TDP-43 (TAR DNA-binding protein) is a DNA- and RNA-binding protein highly conserved in eukaryotes with multiple essential cellular functions in DNA transcription and RNA translation. However, further studies have revealed that TDP-43 is primarily an RNA-binding protein with multiple roles in the regulation of mRNA splicing, translation and transportation, and it is also present in Drosha complex for micro RNA processing and in stress granules for protecting mRNAs in stress conditions. TDP-43 is actually well equipped for RNA binding, as it contains two tandem RNA recognition motifs RRM1 and RRM2, besides the N-terminal domain (NTD) and the C-terminal glycine-rich region. Yet TDP-43 is abnormally aggregated forming inclusions in neuronal cells in amyotrophic lateral sclerosis (ALS) and frontotemporal lobar degeneration (FTLD).

Various DNA and RNA with different sequences and lengths, including TG repeats and UG repeats, were used to co-crystallize with hRRM1, but only a single-stranded 10-nt DNA (5′-GTTGASeGCGTT-3′) with a 2′-methylseleno-adenosine (ASe) could be co-crystallized with hRRM1. The final refined model contained one hRRM1 polypeptide chain (residues 103–179) and one ssDNA (G1 to T9) with an R-factor/R-free of 20.65/25.86% for 4301/430 reflections up to a resolution of 2.75 Å. The overall crystal structure of the hRRM1-DNA complex showed that hRRM1 had an αβ sandwich structure containing a five-stranded β-sheet packed against two α-helices. The ssDNA was bound on the flat surface of the β-sheet of hRRM1 interacting mainly with RNP2 and RNP1 segments. The 5′-end of the DNA extended upward and further interacted with the Loop1 residues. Similar to the classical RRM proteins, the conserved I107 in RNP2 formed nonbonded interactions with C7 and the conserved F149 in RNP1 stacked with G8. Besides stacking with F149, the G8 base also formed hydrogen bonds to hRRM1: N1 and N2 formed hydrogen bonds with residue D105 (Oδ2); N2 formed a hydrogen bond with Q134 (Oε1). G4 inserted into the surface cleft, stacking with W113 (in Loop 1) and R171, and formed extensive hydrogen bonds with hRRM1: N1 and N2 to L111 (backbone O); O6 to W113 (backbone N); N2 to G146 (backbone O); N7 to R171 (Nη1). The long loop, Loop3, interacted with the DNA phosphate backbone of G8, suggesting that it might be crucial for the recognition of the shape but not the sequence of the ssDNA. In summary, hRRM1 bound the ssDNA via nonbonded, π-π stacking interactions and hydrogen bonding, and it might specify the preference for a GC-rich sequence: X-G4-X-G6-C7-G8.

> TSDLIVLGLPWKTTEQDLKEYFSTFGEVLMVQVKKDLKTGHSKGFGFVRFTEYETQVKVMSQRHMIDGRWCDCKLPN>[2x]GSRKIIHVDMDCFFAAVEMRDNPALRDIPIAIGGSRERRGVISTANYPARKFGVRSAMPTGMALKLCPHLTLLPGRFDAYKEASNHIREIFSRYTSRIEPLSLDEAYLDVTDSVHCHGSATLIAQEIRQTIFNELQLTASAGVAPVKFLAKIASDMNKPNGQFVITPAEVPAFLQTLPLAKIPGVGKVSA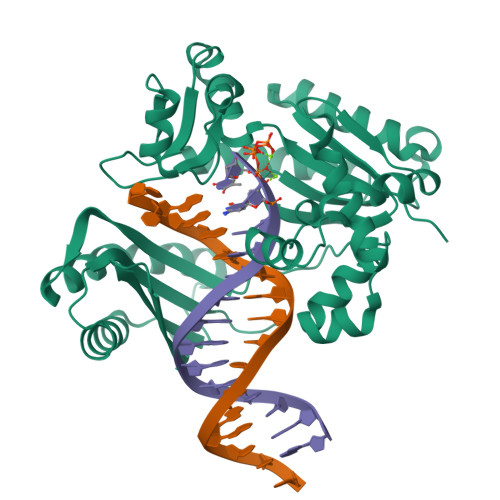AKLEAMGLRTCGDVQKCDLVMLLKRFGKFGRILWERSQGIDERDVNSERLRKSVGVERTMAEDIHHWSECEAIIERLYPELERRLAKVKPDLLIARQGVKLKFDDFQQTTQEHVWPRLNKADLIATARKTWDERRGGRGVRLVGLHVTLLDPQMERQLVLGL> MVLRGVRLRSVAVSCYGSSLTAATRCLSVRTEDFFSKEAISHARRVSWAPHTTEKKQGAFAKLARSNFGDPLPSSFAQEPYFEEEIEAHRKHHRPDV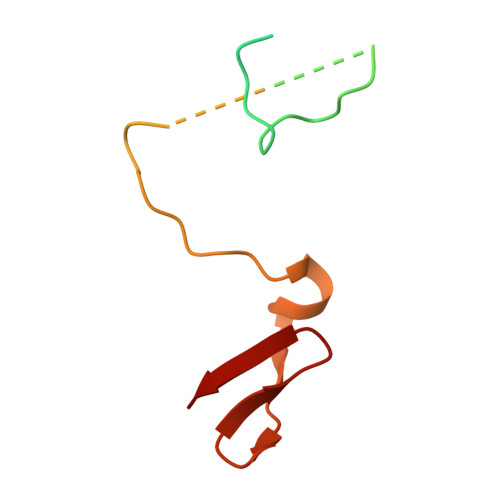YIYKYNVSPTHFSLRE>GSHMDLGFKSGIDLLKQRSTVWKLSTSSSELDSVLGGGLESQSVTEFAGVFGSGKTQIMHQSCVNLQNPEFLFYDEEAVSKGEVAQPKAVYIDTEGTFRPERI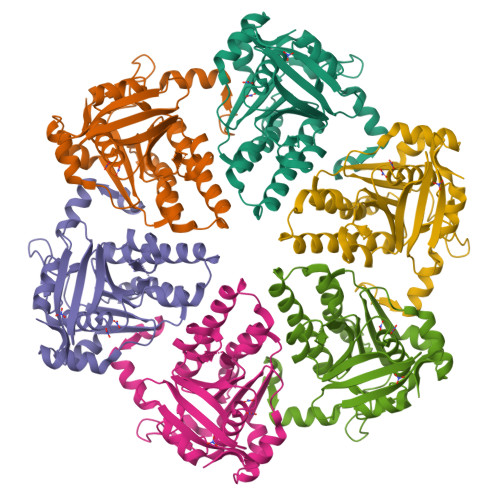MQMAEHAGIDGQTVLDNTFVARAYNSDMQMLFAEKIEDLIQEGNNIKLVVIDSLTSTFRNEYTGRGKLAERQQKLGRHMATLNKLADLFNCVVLVTNQVSAKPDAFFGMAEQAIGGHIVGHAATFRFFVRKGKGDKRVAKLYDSPHLPDAEAIFRITEKGIQD[12x]> MTNTDLKPLLDNLRNATEFWNLVKEASATDESTVHNRSYR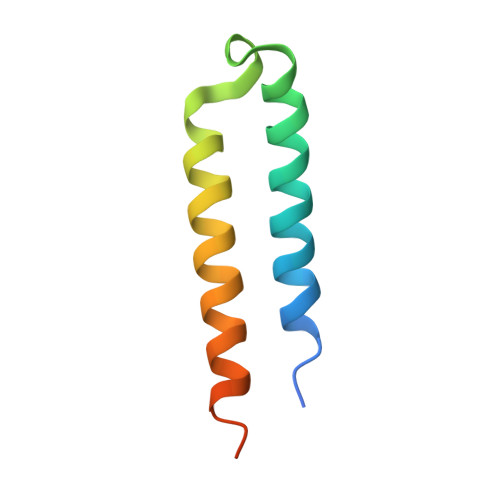DALDWLESAALALGDALIAQRKAVGGDHE>MSLGTYVPGDITLVDSYGNEFQLKNLKGKPIILSPIYTHCRAACPLITKSLLKVIPKLGTPGKDFWVITFTFDPKDTLEDIKRFQKEYGIDGKGWKVVKAKTSEDLFKLLDAIDFRFMTAGNDFIHPNVVVVLSPELQIKDYIYGVNYN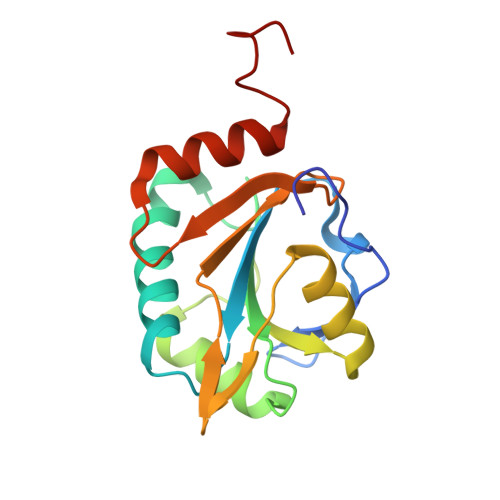YLEFVNALRLARGEGHHHHHH[2x]> MNTRTIYLAGGCFWGLEAYFQRIDGVVDAVSGYANGNTKNPSYEDVSYRHTGHAETVKVTYDADKLSLDDILQYFFR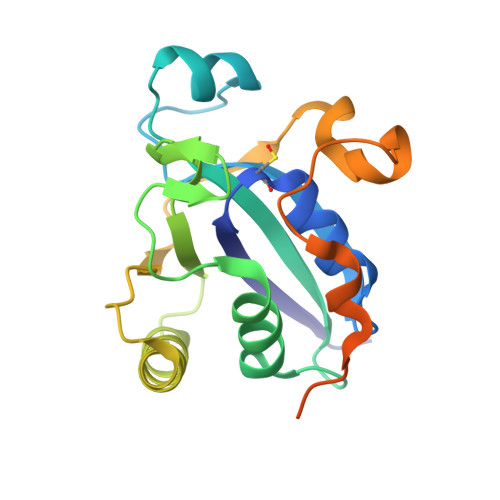VVDPTSLNKQGNDTGTQYRSGVYYTDPAEKAVIAAALKREQQKYQLPLVVENEPLKNFYDAEEYHQDYLIKNPNGYSHIDIRKADEPLPGKTKTAPQGKGFDAATYKKPSDAELKRT>MATPRGLGALLLLLLLPTSGQEKPTEGPRNTCLGSNNMYDIFNLNDKALCFTKCRQSGSDSCNVENLQRYWLNYEAHLMKEGLTQKVNTPFLKALVQNLSTNTAEDFYFSLEPSQVPRQVMKDEDKPPDRVRLPKSLFRSLPGNRSVVRLAVTILDIGPGTLFKGPRLGLGDGSGVLNNRLVGLSVGQM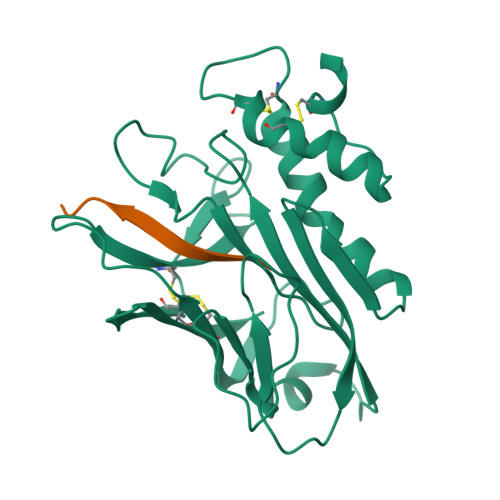HVTKLAEPLEIVFSHQRPPPNMTLTCVFWDVTKGTTGDWSSEGCSTEVRPEGTVCCCDHLTFFALLLRPTLDQSTTKHHHHHH[4x]Given the auxotrophic nature of pneumococci for certain amino acids, the Ami ABC transporter system, orchestrating oligopeptide uptake, becomes indispensable in host compartments lacking amino acids. The system comprises five exposed Oligopeptide Binding Proteins (OBPs) and four proteins building the ABC transporter channel. Crucially, SBPs determine the specificity of their respective transport systems, thereby governing the range of molecules capable of entering the cell. The five lipoproteins exhibit pairwise sequence identity of ~52–60% and share a very similar overall folding.

To evaluate AliB’s capacity to recognize diverse peptides, the protein was incubated with an excess of defined synthesized peptides (peptides 2, 3 and 4) that were previously reported to bind AliB. Specifically, crystal structures of AliB in complex with peptide 2 (AIQSEKARKHN), peptide 3 (PIVGGHEGAGV), and peptide 4 (VMVKGPGPGREST) were solved at resolutions of 2.29 Å, 1.66 Å and 1.49 Å, respectively. Peptide 3, comprising 11 residues (PIVGGHEGAGV), shares the same length as peptide 2, but possesses a distinctly different sequence. Analogous to peptide 2, the initial three residues adopt a short β-strand conformation. However, in contrast to peptide 2, the subsequent portion of peptide 3 lacks a substantial quantity of basic residues, comprising several glycines and other non-bulky residues. In this case, the ligand inside the AliB binding-site does not exhibit any secondary structural elements except for the conserved β-strand at the N-terminus. The two glycine (G) residues in the peptide (residues 4 and 5) do not engage in polar interactions with AliB, while the following two G residues (residues 8 and 10) establish strong stabilizing H-bonds. Particularly noteworthy are the salt-bridge interactions that take place between peptide 3 and AliB (H6 from the substrate with E440 from AliB, and E7 from the substrate with K437 and H497 from AliB). Additionally, a few other H-bond contacts are observed with the last four residues of the substrate (GAGV).

>NSSTASKTYNYVYSSDPSSLNYLAENRAATSDIVANLVDGLLENDQYGNIIPSLAEDWTVSQDGLTYTYKLRKDAKWFTSEGEEYAPVTAQDFVTGLQYAADKKSEALYLVQDSVAGLDDYITGKTSDFSTVGVKALDDQTVQYTLVKPELYWNSKTLATILFPVNADFLKSKGDDFGKADPSSILYNGPFLMKALVSKSAIEYKKNPNYWDAKNVFVDDVKLTYYDGSDQESLERNFTAGAYTTARLFPNSSSYEGIKEKYKNNIIYSMQNSTSYFFNFNLDRKSYNYTSKTSDIEKKSTQEAVLNKNFRQAINFAFDRTSYGAQSEGKEGATKILRNLVVPPNFVSIKGKDFGEVVASKMVNYGKEWQGINFADGQDPYYNPEKAKAKFAEAKKELEAKGVQFPIHLDKTVEVTDKVGIQGVSSIKQSIESVLGSDNVVIDIQQLTSDEFDSSGYFAQTAAQKDYDLYHGGWGPDYQDPSTYLDIFNTNSGGFLQNLGLEPGEANDKAKAVGLDVYTQMLEEANKEQDPAKRYEKYADIQAWLIDSSLVLPSVSRGGTPSLRRTVPFAAAYGLTGTKGVESYKYLKVQDKIVTTDEYAKAREKWLKEKEESNKKAQEELAKHVK[2x];>[2x]PIVGGHEGAGV>GNSEEDYPNGTWLGDENNPEMRVRCAIIPSDMLHISTNCRTAEKMALTLLDYLFHR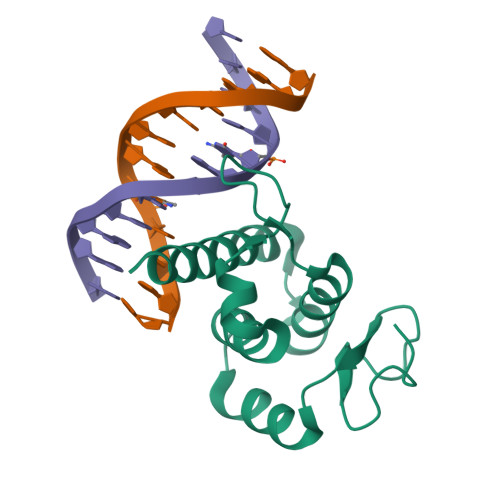EVQAVSNLSGQGKHGKKQLDPLTIYGIRCHLFYKFGITESDWYRIKQSIDSKCRTAWRRKQRGQSLAVKSFSRRTPNSSSYCPSE[2x]>[2x]MGSDKIHHHHHHMRKAW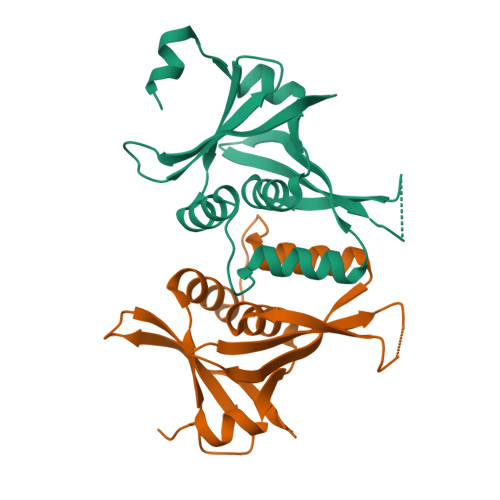VKTLALDRVSNTPVVILGIEGTNRVLPIWIGAAEGHALALAMEKMEFPRPLTHDLLLSVLESLEARVDKVIIHSLKDNTFYATLVIRDLTYTDEEDEEAALIDIDSRPSDAIILAVKTGAPIFVSDNLVEKHSIELEVNERDLINSR> GAMDGTAAEPRPGAGSLQHAQPPPQPRKKRPEDFKFGKILGEGSFSTVVLARELATSREYAIKILEKRHIIKENKVPYVTRERDVMSRLDHPFFVKLYFTFQDDEKLYFGLSYAKNGELLKYIRKIGSFDETCTRFYTAEIVSALEYLHGKGIIHRDLKPENILLNEDMHIQITDFGTAKVLSPESKQARANSFVGTAQYVSPELLTEKSACKSSDL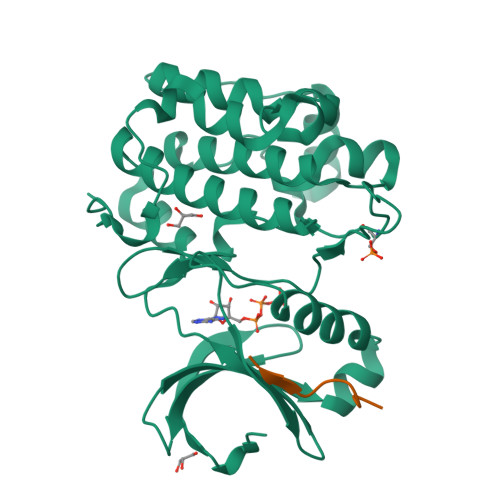WALGCIIYQLVAGLPPFRAGNEGLIFAKIIKLEYDFPEKFFPKARDLVEKLLVLDATKRLGCEEMEGYGPLKAHPFFESVTWENLHQQTPPKLT;> EEQEMFRDFDYIADW2-(5-chlorothiophen-2-yl)-N-[(3S)-1-(4-{2-[(dimethylamino)methyl]-1H-imidazol-1-yl}-2-fluorophenyl)-2-oxopyrrolidin-3-yl]ethanesulfonamide | 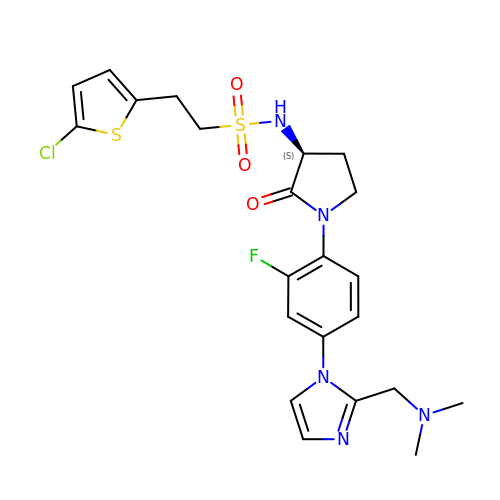C22 H25 Cl F N5 O3 S2 | JENHCPNBBPPGMN-SFHVURJKSA-N>MSKRLRVEDDFNPVYPYGYARNQNIPFLTPPFVSSDGFQNFPPGVLSLKLADPIAIANGNVSLKVGGGLTVEQQSGKLSVDTKAPLQVANDNKLELSYDDPFKVENNKLGIKAGHGLAVVTKENTSLPSLVGTLVVLTGKGIGTGSSAHGGTIDVRLGEGGGLSFDEKGDLVAWDKKNDTRTLWTTPDPSPNCKVETARDSKLTLALTKCGSQILATVSLLVVTGKYAIISDTVNPKQFSIKLLFNDKGVLLSDSNLDGTYWNYRSNNNNIGTPYKEAVGFMPSTTAYPKPTNNTSTDPDKKVSQGKN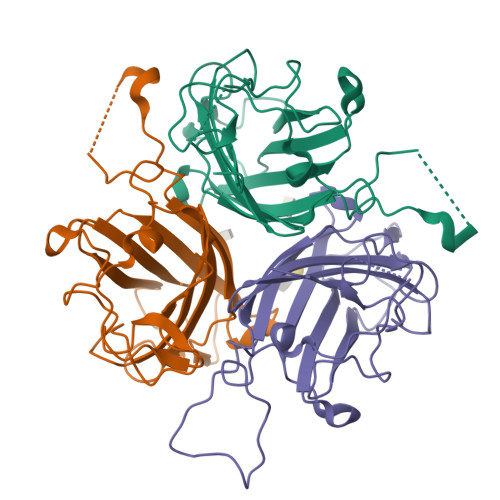KIVSNIYLGGEVYQPGFIVVKFNQETDANCAYSITFDFGWGKVYKDPIPYDTSSFTFSYIAQE[3x]>MTTGKPNILIIMVDQLNGKLFPDGPADFLHAPNLKALAKRSARFHNNYTSSPLSAPARASFMAGQLPSRTRVYDNAAEYQSSIPTYAHHLRRAGYYTALSGKMHLVGPDQLHGFEERLTTDIYPADFGWTPDYRKPGERIDWWYHNLGSVTGAGVAEITNQMEYDDEVAFLANQKLYQLSRENDDESRRPWCLTVSFTHPHDPYVARRKFWDLYEDCEHLTPEVGAIPLDEQDPHSQRIMLSCDYQNFDVTEENVRRSRRAYFANISYLDEKVGELIDTLTRTRMLDDTLILFCSDHGDMLGERGLWFKMNFFEGSARVPLMIAGPGIAPGLHLTPTSNLDVTPTLADLAGISLEEVRPWTDGVSLVPMVNGVERTEPVLMEYAAEASYAPLVAIREGKWKYVYCALDPEQLFDLEADPLELTNLAENPRGPVDQATLTAFRDMRAAHWDMEAFDAAVRESQARRWVVYEALRNGAYYPWDHQPLQKASERYMRNHMNLDTLEESKRYPRGEGSHHHHHH[4x]

Choline-O-sulfatase (COSe; EC 3.1.6.6) is a member of the alkaline phosphatase (AP) superfamily, and its natural function is to hydrolyze choline-O-sulfate into choline and sulfate. Choline-O-sulfatase (COSe; EC 3.1.6.6) is responsible for the first step of this pathway, consisting of the breakdown of COS into choline. This enzyme belongs to the S1 family of sulfatases (subfamily 12) according to the SulfAtlas database. Like other arylsulfatases and phosphonate monoester hydrolases (PMHs; van Loo et al., 2010, van Loo, Bayer et al., 2019), SmeCOse is a mononuclear metalloenzyme. DLS experiments performed at pH 8.0 show a single peak in the particle-size distribution by intensity, with a hydrodynamic radius of 5.7 ± 2.1 nm, which corresponds to a globular protein size of 200 kDa, also supporting a tetrameric quaternary arrangement.

The COSe from S. meliloti CECT4857 used in this work presents a single L105F mutation with respect to that protein (Genbank Accession No. QAT12853). WT SmeCOSe crystals alone or co-crystallized with choline were grown in 1.0 M Li2SO4, 0.1 M Tris pH 7.0, whereas the HEPES-bound C54S SmeCOSe structure was obtained from crystals obtained using 1.5 M Li2SO4, 0.1 M HEPES pH 7.5; they belonged to space group C121. The largest shift of Tyr123 occurs in the HEPES-bound structure and might be attributed to the bulkier piperazine ring compared with the methyl groups of choline. Lys102 (representing Lys A in other sulfatases; Hanson et al., 2004) is also displaced, but only in the HEPES-bound C54S structure.>MAHHHHHHMKNIIITGGAGFIGSHVVREFVIKNPEITIINLDALTYAGNLENLKDIENFPNYVFEKADITKPEELRKVFEKYNPDAVVHLAAESHVDRSITDPNAFINTNVIGTANLLNLCREFWTLNPEHTHGRFPNEPRTNLFYHVSTDEVYGSLGETGFFLETTAYDPQSPYSASKAASDHLVRAYGNTYGMPFIVSNCSNNYGPNHFPEKLIPLCISNILNEKPLPIYGDGKYTRDWLYVIDHARAIHQIFNE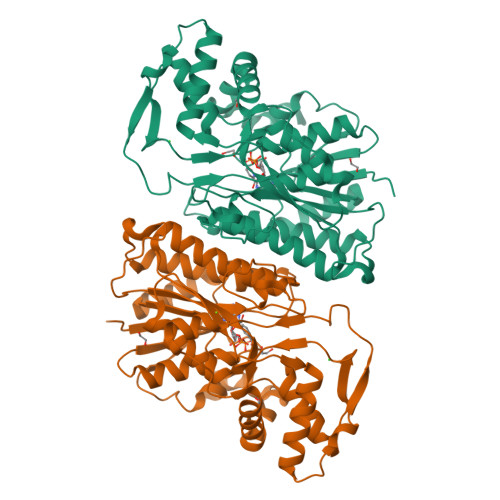AKTGETYNIGGFNEWQNIDLVKELIKQLDAKLGKPEGHSEKLITFVKDRPGHDKRYAIDATKLNKDLGWKPSVTFEEGLAKTIDWYLDNKEWLENVTSGDYQKYYENQYS[4x]As a broad spectrum and readily transferable MBL, NDM-1 confers resistance to nearly all β-lactam antibiotics in a wide range of Gram-negative pathogens. NDM-1 has broad specificity with kcat/KM values of 106–107 M−1 s−1 for hydrolysis of penicillins, cephalosporins, and carbapenems. Other than the ligands for the active site Zn ions, the active site of NDM-1 is composed largely of hydrophobic residues. Lys224 and Asn233 are the only residues that make polar interactions with the antibiotic substrate.

Further combining the substitutions resulted in a triple mutant, K224R/G232A/N233Q, which is as active as the wild-type enzyme in hydrolyzing AMP but exhibits a 600-fold reduction in kcat/KM for IMP hydrolysis. In order to understand the basis for its altered substrate specificity, the structure of the triple mutant was determined by X-ray crystallography to 1.75 Å resolution with four molecules in the asymmetric unit. In each chain of NDM-1 K224R/G232A/N233Q, there are zinc ions coordinated to the histidine site and cysteine site. A water molecule or hydroxide ion was found between the two zinc ions in each chain. The K224R/G232A/N233Q mutations do not result in large changes in the overall structure of NDM-1 but do cause a large change in the conformation of loop L10 where the mutations occur. Specifically, although the side chain of Arg224 in NDM-1 K224R/G232A/N233Q chain A has a similar orientation as that of Lys224 in the wild-type protein, the side chain of Gln233 in the mutant adopts a very different orientation from that of Asn233 in the wild-type enzyme and is pointed out of the active site. The main chain conformation of the triple mutant is drastically altered between Ala232 and Asp236. This has the effect of placing the side chain of Leu234 of the mutant in the position of Asn233 in wild-type and the side chain of Gln233 of the mutant in the position of Leu234 in wild-type. As Asn233 in wild-type NDM-1 is predicted to form a hydrogen bond with the carboxylate group of the reaction intermediate of β-lactams, this interaction would be abolished in the K224R/G232A/N233Q mutant, with the Asn233 hydrogen-bonding group replaced by the Leu234 hydrophobic group. In addition, the methyl group of Ala232 in the mutant protein protrudes toward the active site, which may cause steric clash with β-lactams with bulky R2 groups such as cephalosporins and carbapenems.

>ETGDQRFGDLVFRQLAPNVWQHTSYLDMPGFGAVASNGLIVRDGGRVLVVDTAWTDDQTAQILNWIKQEINLPVALAVVTHAHQDKMGGMDALHAAGIATYANALSNQLAPQEGMVAAQHSLTFAANGWVEPATAPNFGPLKVFYPGPGHTSDNITVGIDGTDIAFGGCLIRDSKAKSLAQLGDADTEHYAASARAFGAAFPKASMIVMSHSAPDSRAAITHTARMADKLR[4x]> XGAAQ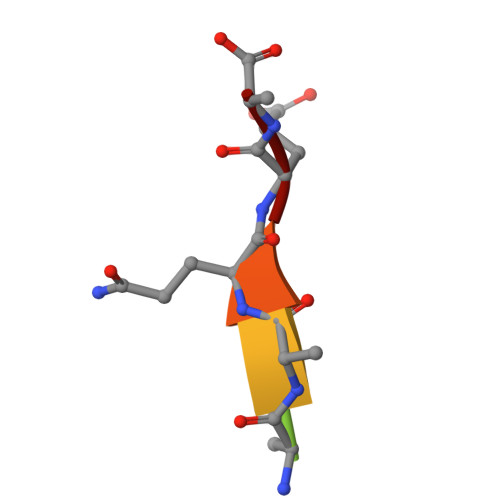EE> MLPFLLATLGTTALNNSNPKDYCYSARIRSTVLQGLPFGGVPTVLALDFMCFLALLFLFSILRKVAWDYGRLALVTDADRLRRQERDRVEQEYVASAMHGDSHDRYERLTSVSSSVDFDQRDNGFCSWLTAIFRIKDDEIRDKCGGDAVHYLSFQRHIIGLLVVVGVLSVGIVLPVNFSGDLLENNAYSFGRTTIANLKSGNNLLWLHTSFAFLYLLLTVYSMRRHTSKMRYKEDDLVKRTLFINGISKYAESEKIKKHFEEAYPNCTVLEARPCYNVARLMFLDAERKKAERGKLYFTNLQSKENVPTMINPKPCGHLCCCVVRGCEQVEAIEYYTKLEQKLKEDYKREKEKVNEKPLGMAFVTFHNETITAIILKDFNVCKCQGCTCRGEPRPSSCSESLHISNWTVSYAPDPQNIYWEHLSIRGFIWWLRCLVINVVLFILLFFLTTPAIIITTMDKFNVTKPVEYLNNPIITQFFPTLLLWCFSALLPTIVYYSAFFEAHWTRSGENRTTMHKCYTFLIFMVLLLPSLGLSSLDLFFRWLFDKKFLAEAAIRFECVFLPDNGAFFVNYVIASAFIGNAMDLLRIPGLLMYMIRLCLARSAAERRNVKRHQAYEFQFGAAYAWMMCVFTVVMTYSITCPIIVPFGLMYMLLKHLVDRYNLYYAYLPAKLDKKIHSGAVNQVVAAPILCLFWLLFFSTMRTGFLAPTSMFTFVVLVITIVICLCHVCFGHFKYLSAHNYKIEHTETDTVDPRSNGRPPTAAAVPKSAKYIAQVLQDSEVDGDGDG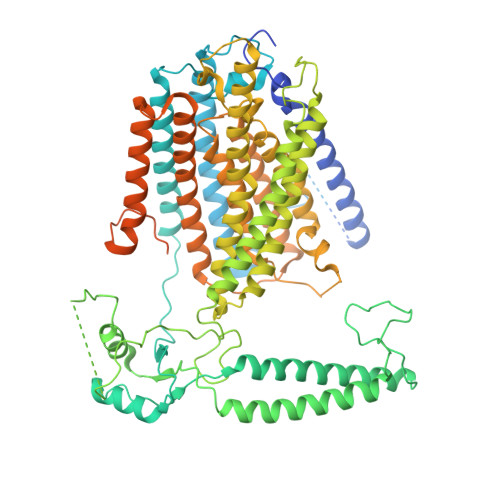APGSSGDEPPSSSSQDEELLMPPDALTDTDFQSCEDSLIENEIHQSNSWSHPQFEKL>[2x]SIKIECVLPENCRCGESPVWEEVSNSLLFVDIPAKKVCRWDSFTKQVQRVTMDAPVSSVALRQSGGYVATIGTKFCALNWKEQSAVVLATVDNDKKNNRFNDGKVDPAGRYFAGTMAEETAPAVLERHQGALYSLFPDHHVKKYFDQVDISNGLDWSLDHKIFYYIDSLSYSVDAFDYDLQTGQISNRRSVYKLEKEEQIPD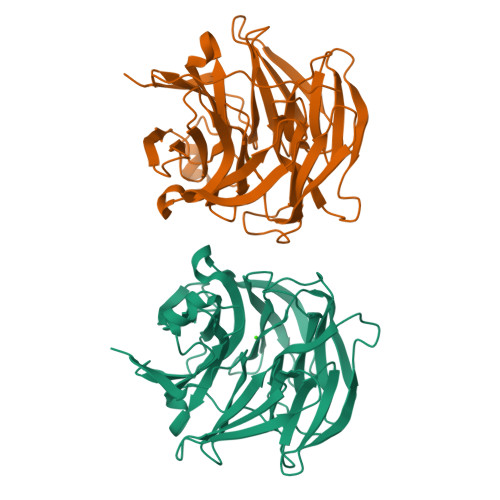GMCIDAEGKLWVACYNGGRVIRLDPVTGKRLQTVKLPVDKTTSCCFGGKNYSEMYVTCARDGMDPEGLLRQPEAGGIFKITGLGVKGIAPYSYAG>[2x]PQFSLWKRPVVTAYIEGQPVEVLLDTGADDSIV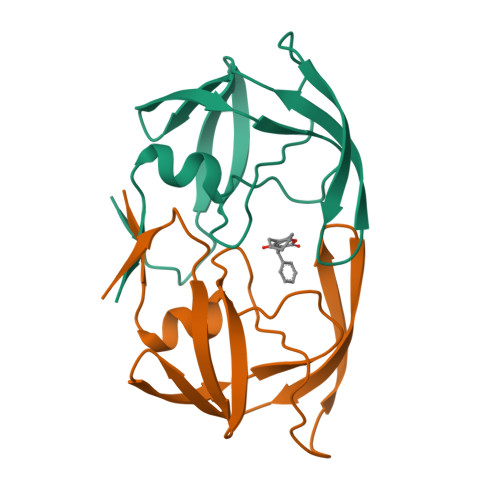AGIELGNNYSPKIVGGIGGFINTLEYKNVEIEVLNKKVRATIMTGDTPINIFGRNILTALGMSLNL>[2x]AIERTLSIIKPDGLEKGVIGKIISRFEEKGLKPVAIRLQHLSQAQAEGFYAVHKARPFFKDLVQFMISGPVVLMVLEGENAVLANRDIMGATNPAQAAEGTIRKDFATSIDKNTVHG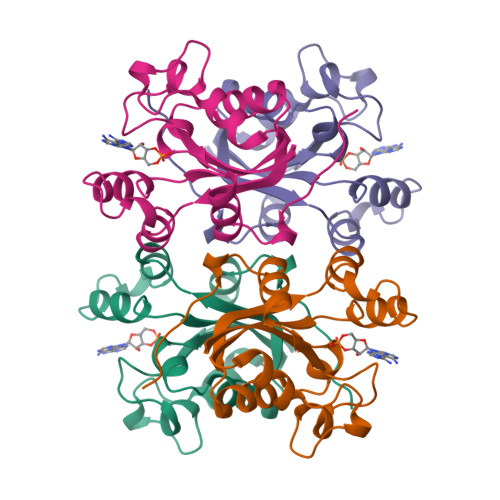SDSLENAKIEIAYFFRETEIHSYPYQK>METTVLVTFEQRLTTGDVGKLSRLIGAVIPIPYRHHLLGSSQVGLDAVVKDKTRDYSRMRARMREMTLTIMRRVEGNQMILGVPTHGQCYTIRNTGPVSWEKGDVLTTLPPVFSGEVTGLVSVSDWDLVLPWIVPMALATEINQRMMMLALLSLDRSHEEVRAATAQLRVVRYRDATLTLPEITIDDTVLIDMRNVCISLSMIANLSSEVTLAYVRKLALEDSNMLLMKCQEILGRRMPQVGVGAGSSGDRNDPPARSRTNYNITPTEELNKLTALFVMIRQITDVISEQPAFLVCDVSPDDKSALCIYKG[10x];>MSARGRAAGDDGRQAELMATLGFVRLSKSSVGKVKKFLNNLYDLKSINLCRHPRVIAECRGTDLSRETQLYNEMVLWLRYHEKLTARRPGHLPLLTRIRQDYDKLFGFVAARPELCGFDGLTEVNVFDDAVYGDDYVPRVDVFLRGLEDLARCLCAQGPDKPARAVIMGFINMRAEEVNRLMDNVRDAAERVLVYEVLDVRDPLNEDPSVLVHNRLVYLCRLAYAISKSWQTLSHMCLDRINSLRRRLILAFHDRPAFARVYARNALERPVDGTTAYNLLRRLEEDFLLFRNALRWGDPDWGLESELESEGDNSDAGSDLDLEDEEDDDDGGGPGGHDDESGGNRTPDPGMSLHDDTGIANTCLIGGDDEDCGGGSGRCLEFDPDSERCLGVKMVNGRALRWWNPTGIMVDNEAAVWIDEHGRVMDKPPPKELRKASSDDGGNKKNPPPKKNVTPPVSGSNSVGGGVQTPSTASGKRTGKKKEGGGGYLLRSRSTDDDEVRKMKKDGTIDDRADRELKMALQKARESTADSDLSTILPRTEPLRKVAFVGDPVAAFGDTVRTTSSSKGFDDGPFTTQGASVLLPPPLGGPGSTLTLPPDLPDLSGVLADEDVQDSRYGKIPKSRTKKHPTFPENYKQRPPPHNKDDEYYWDETGDNMPVGEDGGGVLEDLRKGLEGIDLKTGGGGSLQPPLSQQFAGSPFAGSDGDGGGLVKKSSSSH[8x];>[16x]MGENWTATELLPKLDVPIDLLTHIKLSVGEEMFNNFRLYYGDDPERYNLSFEAIFGTYCNKIEWVTFLGTALATAAHAIMFHDLNKMTTGKMLFYIQVPRVATGAGIPTSRQTTVMVSKYSEKSPITIPFEISAACLTHLKETFEDTLLDKLLNADAVNTVLRAVKNTADAMERGLIDTFLRVLLRHAPPCFVLRTLMEHGTIARRMATRVQRANIAQGFKSKMLATIFLLDRSRDRGQLTRYLDMLTDCVTESILDNPETYTVGGGERLAGVIVSTHTVVQALLNALGGSIRRTGVKTPASYGKFVLSKENAVTAIAHHAIMADFSQHADRIQQSSQKDLPESQFLDQRLTFTETQMDVLKVGERLVALEHLRKVYKNTDVQDPLERDVELTFYFPVGLHVPSGRAYSTAENKIKLVDTAENQLPTTVYFYNKDRIPQRISHAEALKTLCHPAIHDAGPCLEAFAQAGPPQGDDRVRALCRREFVREHMAHATRRLVHFYQARIDPPRTANEAKHDFSTKEFAKVDNYLLFTELHPFFDFCFHTENGQVRPLCTPRIMVGNLPEALAPADFHDLRAKQALELTKVRAPEGHEATLQVLRASLTDHQYPELFYLIESLIHGDPAAFETGIELVTRCVNNYWRQRGLLAFANSYDMVRLIATRLGDGAVVPAAYTHYRNLLSITRFVARTCELTGLNGRLCDEPLLAYVSALHDPRLWPPFVQALPRNANLVRVVADDVPLDAAHIEERNPGTSDVARMIAMDQAEPLFVDARRTSDEEMVAQKVYYLCLVPAVLNNHACGAGLNLKHLLVKLFYTKFFLTADPDSLTAGEEALTNNPLLAALVRDVATDENVTANQAAEELFHLVAHVPENAQMLEIRAALDPAQRHGAPSAGFESLQHVLYNGFCMTTVPKLLQEYLTVIPFHRFYSDPGLAATANHDIRVFLNDFPQYQRCDGGFPLSPIFAHEYHHWHRTPFSCYSAACAHTLESVLTLAIMHHKMSPVSIAALSRMGLHPGFALTVVRTDTFETDTLLYSTKASTAVIINTPIVTKEDRDINTVFHVSQNINTVEMGLGYGATTCTAHLRRVRSDMGSRMQDLFQVFPMHVYRNEDVDAWVRQATGARRTEVLDSEAISILTFGRKTDKGGPALLHGQRATCEVILTPVSADLEFFRYPNNPRGRSSSMLGVDPYDEDAALATLYDHTSPDPQTFVSTNNPWGSQRGSLGDVIYNTRNREKLGHNPSFYSPCAQFFTTDDIINANKTLFKTVEEYLNRSQDCIHGETDLQYICVEGTNSIVEKPCRFLQEALTQHTGTTQALMESQLKGTSKLGLDETHYGNYSIGETIPLQQSILFNS;>MSTNVSSAASGGGSSGGSSGASSGGGGGGSGGSSKKEEERRKQFGANVLNLAPAMVAQPVISTMIPKYMKMGGHEDKLAYQLDLLRMLSIAKKATVIQ[16x];>[5x]MANVSSFGPMKREVMEFDPEDPYKVSKMRKLERSIAKGYVYGADHQAITARFFVRESLGEVEQKNLGVLMFRLDTGIEMPSTVLVSLFFLSMVAENVSAATKNTLAAIYGREGEAIRTWLRDGAWRLHRVVHPLGCTNSITPGATCLITCSMRGHSYNMLKTEIYPLLVPKEIYLDLDGESTDEIRFVYFVITYDYNSDRQGRPSAFVVVSRITHRHTLINVLRYRFRVSRFHFLNNSISGYGPSTGCLGTLQRLGWFCSRDSRSGIVASRAGQLSVVKLEKFYVDVGPLVEFA

Distinct from other medically important herpesviruses (those responsible for cold sores, genital herpes, shingles and several human cancers), CMV contains an abundant phosphoprotein, pp150, which is a structurally, immunogenically, and regulatorily important tegument protein and a potential drug target. Here, by cryoEM and sub-particle reconstructions, we have obtained structures of the MCMV capsid and its associated pM32 (pp150) at near-atomic resolutions and built their atomic models, the first for any MCMV proteins. The ~5 Å 3D reconstruction shows a highly conserved T = 16 icosahedral virion capsid revealing the molecular boundaries among 12 pentons, 150 hexons, 320 triangular triplexes and 260 pM32 (pp150) dimers, allowing identification of individual molecules. An MCP monomer binds an SCP monomer to form a heterodimer, which constitutes one of the five and six subunits in penton and hexon capsomers, respectively.

The structural components within an asymmetric unit encompass 1/5 of a penton capsomer, 2.5 hexon capsomers (1 P hexon, 1 C hexon, and 1/2 of an E hexon), 5 and 1/3 triplexes/pM32 dimers (Ta, Tb, Tc, Td, Te, and 1/3 Tf). To overcome the aforementioned problem of weakened densities and limited resolutions, we have used a sub-particle reconstruction strategy to obtain structures of the MCMV capsid and its associated pM32 at near atomic resolutions and also built atomic models for tegument protein pM32 and all capsid proteins. In total, we have built atomic models of 55 unique conformers, including 16 MCP, 16 SCP, 5 Tri1, 5 Tri2A, 5 Tri2B and 8 pM32nt, amounting to over 27,000 amino acid residues. As detailed below, the atomic models of pM32 of MCMV and pUL32 of HCMV differ, though those for their capsid proteins are similar, with root-mean-square deviation (RMSD) distances between corresponding capsid protein models ranging from 1.95 to 3.36Å (2.47 Å for penton MCP, 2.09 Å for hexon MCP, 1.95 Å for SCP, 3.36 Å for Tri1, 2.05 Å for Tri2A, and 2.10 Å for Tri2B). All bound pM32s are dimerized in MCMV and can be classified into two types, either pM32-a (cyan) or pM32-b (orange-red), based on their relative locations on the capsid. The subunits of pM32nt dimers cluster on each triplex and lean against two neighboring MCPs. pM32nt-a and pM32nt-b are similar in structure (the magnitude of RMSD is 1.20 Å) and form a “Λ”-shape configuration. Careful comparison of the atomic model of pM32 dimer and the corresponding pUL32 subunits in HCMV (for example, pM32 and pUL32 dimer from triplex Te regions) reveals that 17 residues in the pM32-pM32 interface are within 3 Å of each other, as opposed to only 4 residues at the pUL32-pUL32 interface. The existence of 13 additional residues at the molecular interface of the pM32 dimer indicates a stronger and more rigid pM32-pM32 association than between pUL32-pUL32, which is congruent with the pairwise presence/absence of pM32 subunits on MCMV capsid.> MWAFPERFEGRHVRLEPLALAHLPAFLRHYDPEVYRFLSRAPVAPTEEALRAHLEGLLGEPGRVNWAILFGKEVAGRISVIA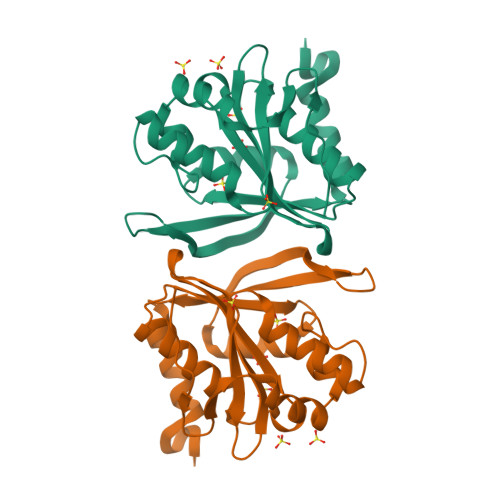PEPEHAKLELGTMLFKPFWGSPANKEAKYLLLRHAFEVLRAERVQFKVDLRNERSQRALEALGAVREGVLRKNRRLPDGAFRDDVVYSVLKEEWPGVKARLEARLYGASGNP>MKITEFMKSKKGASGIGTLIVFIAMVLVAAVAASVLINTSGFLQQKASTTGKESTEQVASGLLINGITGSVGTSDVKLLAIYLAPNAGSSAIDLAQTKVMLDYNGKSVVLGYGGNQDMSSGNSSVFSND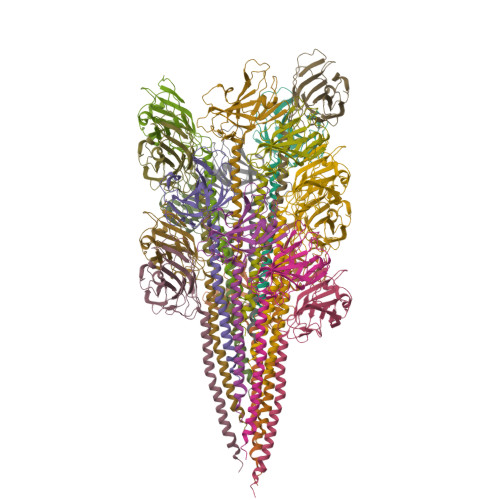TGATATTFQVNILQDYDDSAVDNAVINKGDAVALIVDVNASFAGEIPERTAISGKVQPEFGAPGVISFTTPASYTTTLVELQ[18x]(-)-Isopiperitenone | C10 H14 O 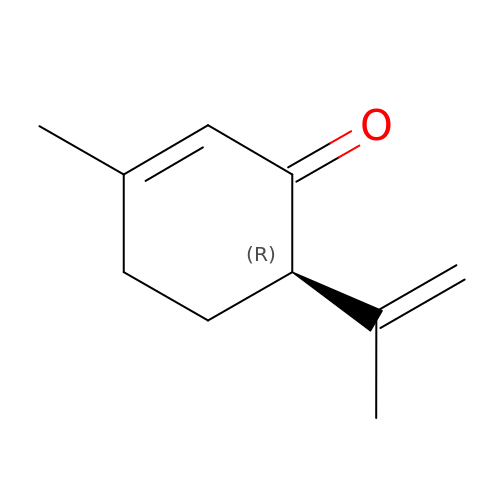| SEZLYIWMVRUIKT-SECBINFHSA-N>[4x]APSMKERQVCCGARDEYWKCLDENLEDASQCKKLRSSFESSCP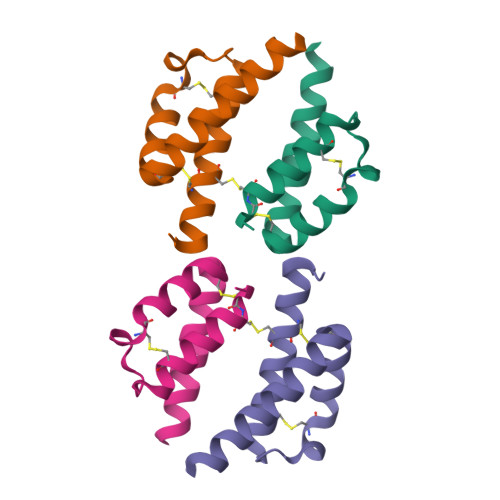QQWIKYFDKRRDYLKFKEKFEA>MVDNSRTRPRVGHIQFLDCLPLYWGLARTGTLLDFELTKDTPEKLSEQLVRGDLDIGPVTLVEFLKNADDLVAFPDIAVGCDGPVMSCVIVSQVPLDRLDGARVALGSTSRTSVRLAQLLLSERFGVQPDYYTCPPDLSLMMQEADAAVLIGDAALRANMIDGPRYGLDVHDLGALWKEWTGLPFVFAVWAARRDYAEREPVITRKVHEAFLASRNLSLEEVEKVAEQAARWEAFDEDTLAK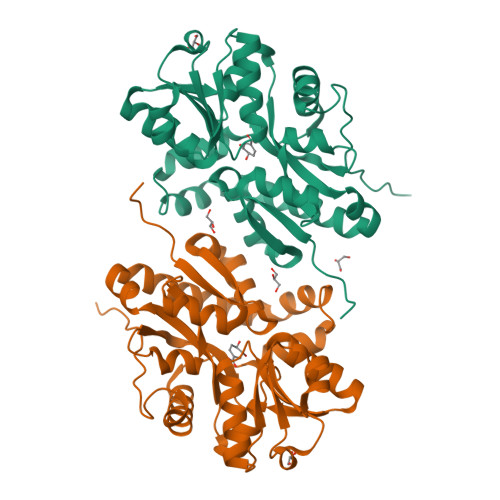YFTTLDFRFGAPQLEAVTEFARRVGPTTGFPADVKVELLKPLEHHHHHH[2x]>[2x]MVKRMIALDGAQGEGGGQILRSALSLSMITGQPFTITSIRAGRAKPGLLRQHLTAVKAATEICGATVEGAELGSQRLLFRPGTVRGGDYRFAIGSAGSCTLVLQTVLPALWFADGPSRVEVSGGTDNPSAPPADFIRRVLEPLLAKIGIHQQTTLLRHGFYPAGGGVVATEVSPVA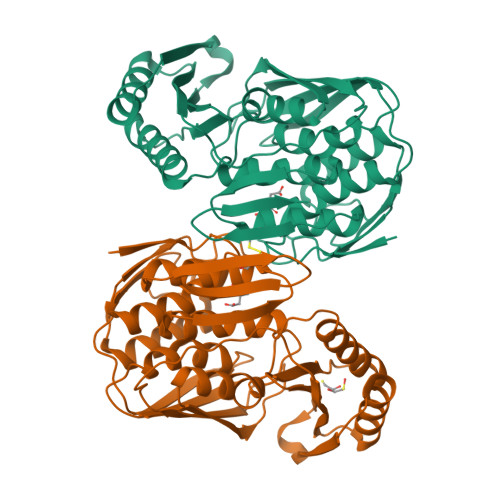SFNTLQLGERGNIVQMRGEVLLAGVPRHVAEREIATLAGSFSLHEQNIHNLPRDQGPGNTVSLEVESENITERFFVVGEKRVSAEVVAAQLVKEVKRYLASTAAVGEYLADQLVLPMALAGAGEFTVAHPSCHLLTNIAVVERFLPVRFSLIETDGVTRVSIEGSHHHHHH> MIKVEIKPSQAQFTTRSGVSRQGKPYSLNEQLCYVDLGNEYPVLVKITLDEGQPAYAPGLYTVHLSSFHVGQFGSL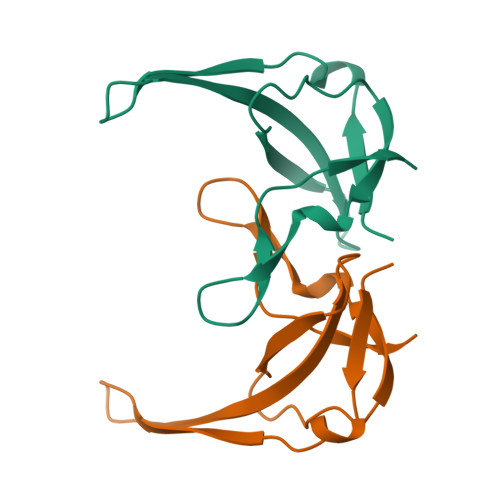MIDRLRLVPAK N-methyl-1-(1-methyl-1H-indazol-3-yl)methanamine 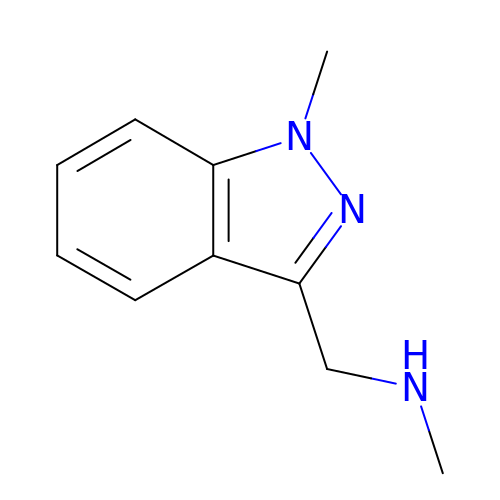| C10 H13 N3 | XDQYKASLVAVERE-UHFFFAOYSA-N> GSHMTRTEIIRELERSLREQEELAKRLKELLRELERLQREGSSDEDVRELLREIKELVEEIEKLAREQKYLVEELKRQQGPPGNEIIRELERSLREQEELA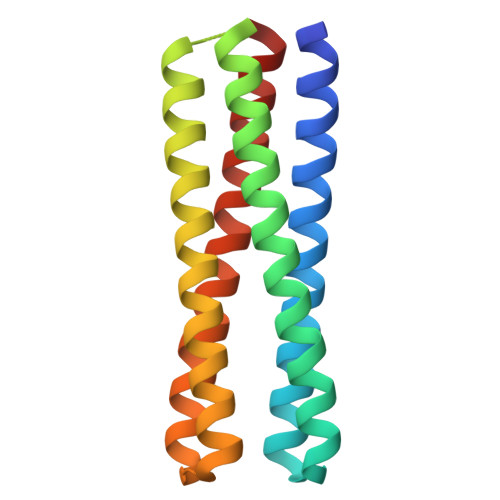KRLKELLRELERLQREGSSDEDVRELLREIKELVEEIEKLAREQKYLVEELKRQD>SLINTKIKPFKNQAFKNGEFIEVTEKDTEGRWSVFFFYPADFVFVCPTELGDVADHYEELQKLGVDVYSVSTDTHFTHKAWHSSSETIAKIKYAMIGDPTGALTRNFDNMREDEGLADRATFVVDPQGIIQAIEVTAEGIGRDASDLLRKIKAAQYVAAHPGEVCPAKWKEG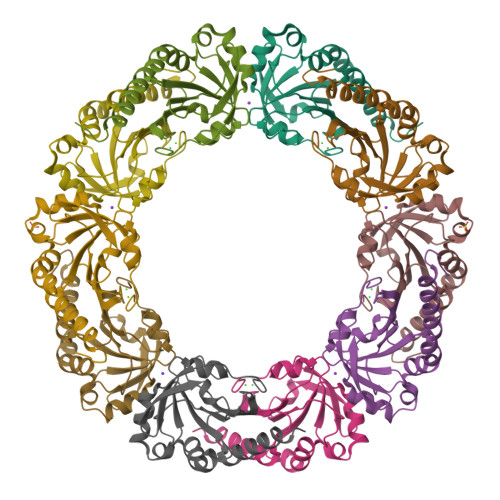EATLAPSLDLVGKI[5x]> MKKLFLVFWWHMHQPLYREPYTGEYLLPWTFFHAVKDYYDMPAYLKDFEIKLNFNLTPVLIDQIQEYAQGKAKDVFLEAIRKDPDDLEKEEVEKLIEFTKLNYEKPIYRFERIRELMNKEKLNREELLDLQTLNLLAWCGRTLRKDLKDLLNKGRNYTQEEKEYVLNKYFEIIKKTLSIYREIKEEGKGSVSTSPYYHPLIPILLNPNCVYETTPNVKIPDFAVSFREDASKHVELAKEKYFEIFGEHPVYMWPPEASVSNEALELYYEKGINMLATDEVILKNSVERASPYLRYYFRELISVFFRDKTLSDLIGFSYHAWNAEDAVRDFIGRLKKIHESVDFQPVVFVVLDGENCWEYYEENGIPFLEKLYSTLEKEEWIETLTLEEAMRKEDVKTEVIESVKAGTWFDGNFLKWIGNKEKNEYWKILIEAKKKAKNDYILVAEGSDWFWWQGEEKAPFVEVFDKLFRSFVRRAQE;> MKKLFLVFWWHMHQPLYREPYTGEYLLPWTFFHAVKDYYDMPAYLKDFEIKLNFNLTPVLIDQIQEYAQGKAKDVFLEAIRKDPDDLEKEEVEKLIEFTKLNYEKPIYRFERIRELMNKEKLNREELLDLQTLNLLAWCGRTLRKDLKDLLNKGRNYTQEEKEYVLNKYFEIIKKTLSIYREIKEEGKGSVSTSPYYHPLIPILLNPNCVYETTPNVKIPDFAV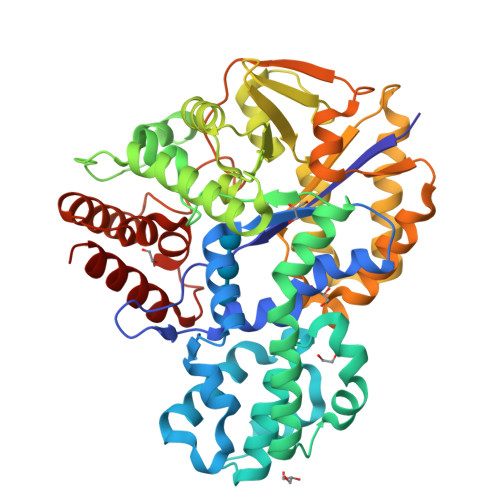SFREDASKHVELAKEKYFEIFGEHPVYMWPPEASVSNEALELYYEKGINMLATDEVILKNSVERASPYLRYYFRELISVFFRDKTLSDLIGFSYHAWNAEDAVRDFIGRLKKIHESVDFQPVVFVVLDGENCWEYYEENGIPFLEKLYSTLEKEEWIETLTLEEAMRKEDVKTEVIESVKAGTWFDGNFLKWIGNKEKNEYWKILIEAKKKAKNDYILVAEGSDWFWWQGEEKAPFVEVFDKLFRSFVRRAQEH(2S)-1-{[(S)-{[(1S,2R,3R,4S,5S,6R)-2-[(6-O-hexadecanoyl-beta-L-gulopyranosyl)oxy]-3,4,5-trihydroxy-6-{[beta-D-mannopyranosyl-(1->2)-alpha-D-mannopyranosyl-(1->6)-beta-D-mannopyranosyl-(1->6)-alpha-D-mannopyranosyl]oxy}cyclohexyl]oxy}(hydroxy)phosphoryl]oxy}-3-(hexadecanoyloxy)propan-2-yl 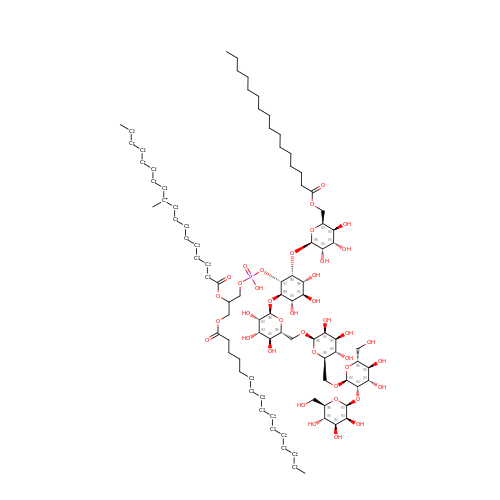10-methyloctadecanoate | C90 H105 O39 P | CVNNFCFROHYSER-GLBWEKRISA-N> RDVQNNIVDEIKYREEVCNDEVDLYLLMDGSGSIRRHNWVNHAVPLAMKLIQQLNLNDNAIHLYASVFSNNAREIIRLHSDASKNKEKALIIIKSLLSTNLPYGKTSLTDALLQVRKHLNDRINRENANQLVVILTDGIPDSIQDSLKESRKLSDRGVKIAVFGIGQGINVAFNRFLVGCHPSDGKCNLYADSAWENVKNVIGPFMKAVCVEVEKTASCGVWDEWSPC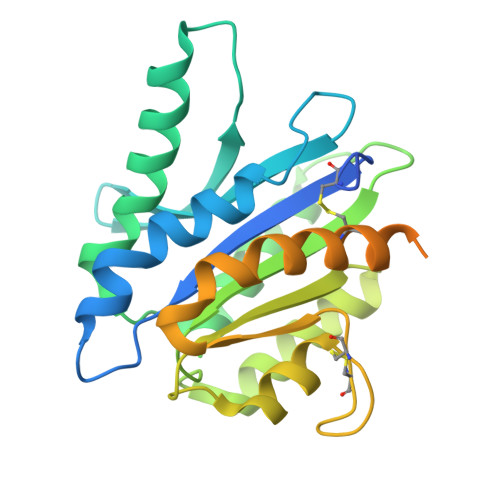SVTCGKGTRSRKREILHEGCTSELQEQCEEERCLPKREPLDVPDEPHHHHHHA>[2x]MGRFVVWPSELDS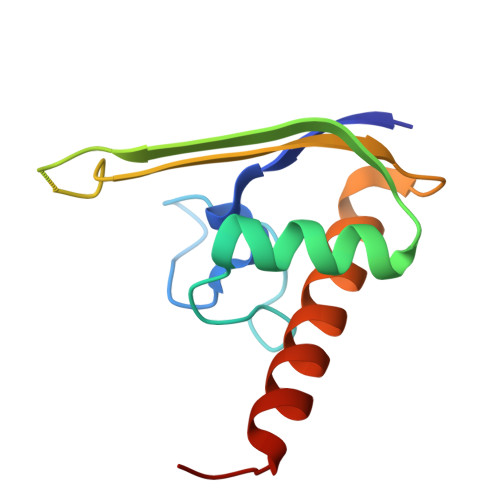RLSRKYGRIVPRSIAVESPRVEEIVRAAEELKFKVIRVEEDKLNPRLSGIDEELRTFGMIVLESPYGKSKSLKLIAQKIREFRRRSAGTLVPR> MCNCCCKGSKDPRFEKVDEILSKLANERGALIAILQHVQHEFGYLPEDVIFYIASKTGIPASKIYGVATFYAQFHLKPRGKYVIRVCLGTACHVKGANKILAEFEKQLGIKAGETTS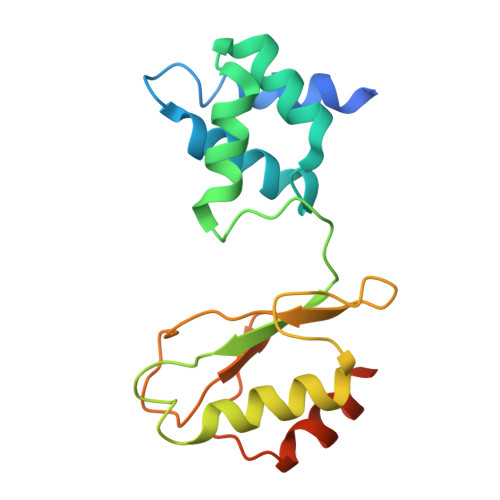DLKFTLERVGCLGACGLAPTVMVNEKTYGKMTPEKVSEVLKEYSDVEAAASAQ>[2x]MAVTLDKDAYYRRVKRLYSNWRKGEDEYANVDAIVVSVGVDEEIVYAKSTALQTWLFGYELTDTIMVFCDDKIIFMASKKKVEFLKQIANTKGNENANGAPAITLLIREKNESNKSSFDKMIEAIKESKNGKKIGVFSKDKFPGEFMKSWNDCLNKEGFDKIDISAVVAYTIAVKEDGELNLMKKAASITSEVFNKFFKERVMEIVDADEKVRHSKLAESVEKAIEEKKYLAGADPSTVEMCY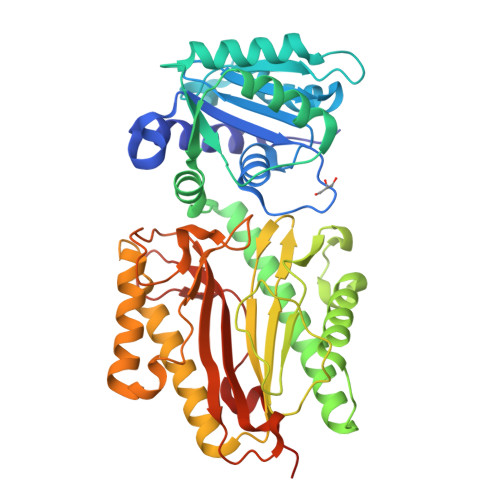PPIIQSGGNYNLKFSVVSDKNHMHFGAITCAMGIRFKSYCSNLVRTLMVDPSQEVQENYNFLLQLQEELLKELRHGVKICDVYNAVMDVVKKQKPELLNKITKNLGFGMGIEFREGSLVINSKNQYKLKKGMVFSINLGFSDLTNKEGKKPEEKTYALFIGDTVLVDEDGPATVLTSVKKKVKNVGIFLKNEDE(5S)-5-methyloxolane-2,2-diol 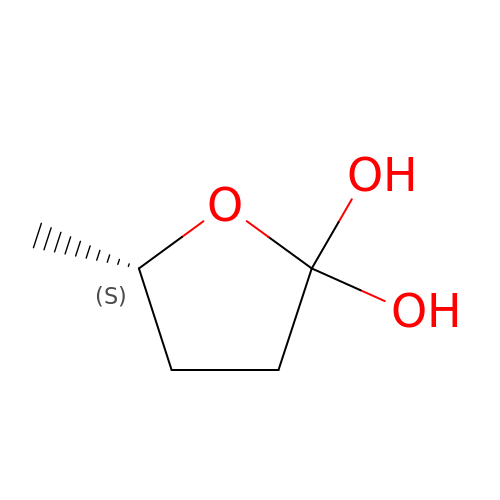| C5 H10 O3 | MGKWNPVXYGZJRN-BYPYZUCNSA-N>[6x]GANAMAHMGKTLRFEIVSGVNKGYFHTNSQSESLDLVGGIWQKIAKEEFEKSNIYVSAVIKPSKTVYNQEWGCPENGQETVVLTGVANEEFVDDIEKWKDTVIKLAKELKNQMKQSTLTCEFIETELHYFK

Although most signal via cyclic oligoadenylate, an alternative class of signalling molecule SAM-AMP, formed by conjugating ATP and S-adenosylmethionine, was described recently. SAM-AMP activates a trans-membrane effector of the CorA magnesium transporter family to provide anti-phage defence. NrN is replaced by a SAM-AMP lyase in some CorA-associated type III CRISPR systems, including that from Clostridium botulinum. SAM-AMP lyase exhibits a typical trimeric PII-like protein architecture characterized by a triangular core formed by the four-stranded antiparallel β-sheet of each subunit.

Crystals of the E71Q variant, targeting a key predicted active site residue, were soaked with SAM-AMP prior to vitrification and data collected to 1.65 Å resolution. Although SAM-AMP lyase E71Q variant crystals were soaked with SAM-AMP, the product following cleavage, MTA-AMP, was observed in the maximum likelihood/σA weighted Fobs–Fcalc electron density map at 3σ, indicating turnover had occurred. MTA-AMP binds at the interface between two monomers in the trimeric complex. Several residues on the T-loop (comprising residues 59–71) and B-loop (comprising residues 106–111) of SAM-AMP lyase constitute the binding site for MTA-AMP. The adenine base of AMP is stabilized by π-stacking interactions with the side chains of W64 and F84. T110 and Y122 form hydrogen bonds with the bridging phosphate moiety and the adenine base of MTA interacts with T112 and S50. Note that of the residues discussed, F84, Y122, S50, Y48, and N81 are from a different subunit to the others, demonstrating the significant contributions of neighbouring monomers to ligand binding. The crystal structure of MTA-AMP bound in SAM-AMP lyase confirms the predicted 3′–5′ phosphodiester bond between the SAM and AMP moieties formed by Cas10. MTA-AMP is buried in a ‘slot-like’, predominantly electronegative, cleft between the subunits of SAM-AMP lyase, with the predicted position of the carboxyl group in the substrate SAM-AMP orientated towards the B-loop. There is an extended binding site for the AMP moiety, which affords SAM-AMP lyase specificity for SAM-AMP over SAM, which is not a substrate.>[4x]MSIPETQKGVIFYESHGKLEYKDIPVPKPKANELLINVKYSGVCHTDLHAWHGDWPLPTKLPLVGGHEGAGVVVGMGENVKGWKIGDYAGIKWLNGSCMACEYCELGNESNCPHADLSGYTHDGSFQEYATADAVQAAHIPQGTDLAEVAPVLCAGITVYKALKSANLMAGHWVAISGAAGGLGSLAVQYAKAMGY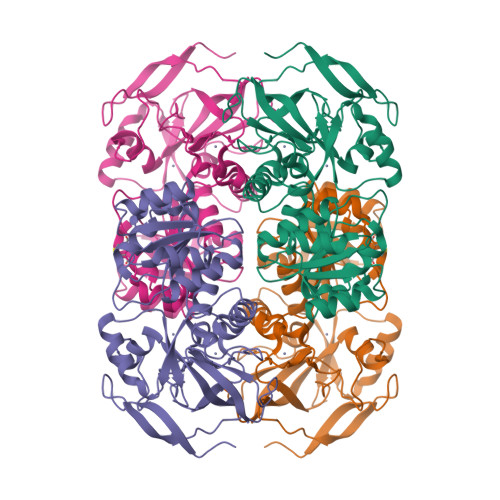RVLGIDGGEGKEELFRSIGGEVFIDFTKEKDIVGAVLKATDGGAHGVINVSVSEAAIEASTRYVRANGTTVLVGMPAGAKCCSDVFNQVVKSISIVGSYVGNRADTREALDFFARGLVKSPIKVVGLSTLPEIYEKMEKGQIVGRYVVDTSK> MNTTTYDYIVVGGGTSGLVVANRLSENPDVSVLLLEAGASVFNNPDVTNANGYGLAFGSAIDWQYQSINQSYAGGKQQVLRAGKALGGTSTINGMAYTRAEDVQIDVWQKLGNEGWTWKDLLPYYLKSENLTAPTSSQVAAGAAYNPAVNGKEGPLKVGWSGSLASGNLSVALNRTFQAAG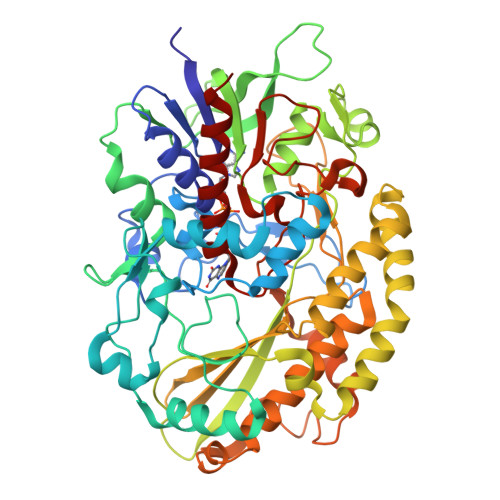VPWVEDVNGGKMRGFNIYPSTLDVDLNVREDAARAYYFPYDDRKNLHLLENTTANRLFWKNGSAEEAIADGVEITSADGKVTRVHAKKEVIISAGALRSPLILELSGVGNPTILKKNNITPRVDLPTVGENLQDQFNNGMAGEGYGVLAGASTVTYPSISDVFGNETDSIVASLRSQLSDYAAATVKVSNGHMKQEDLERLYQLQFDLIVKDKVPIAEILFHPGGGNAVSSEFWGLLPFARGNIHISSNDPTAPAAINPNYFMFEWDGKSQAGIAKYIRKILRSAPLNKLIAKETKPGLSEIPATAADEKWVEWLKANYRSNFHPVGTAAMMPRSIGGVVDNRLRVYGTSNVRVVDASVLPFQVCGHLVSTLYAVAERASDLIKEDAKSA>[2x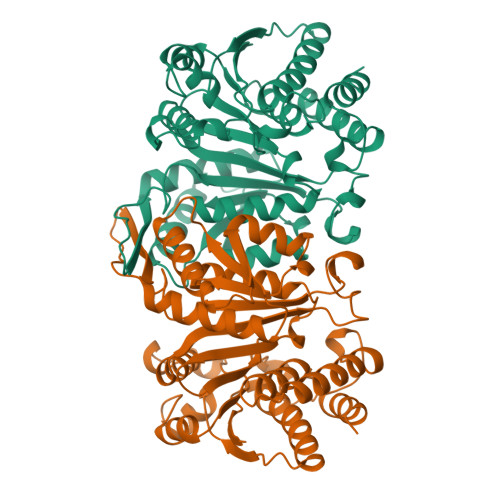]MKVAVLPGDGIGPEVTEAALKVLRALDEAEGLGLAYEVFPFGGAAIDAFGEPFPEPTRKGVEEAEAVLLGSVGGPKWDGLPRKIRPETGLLSLRKSQDLFANLRPAKVFPGLERLSPLKEEIARGVDVLIVRELTGGIYFGEPRGMSEAEAWNTERYSKPEVERVARVAFELARKRRKHVVSVDKANVLEVGEFWRKTVEEVGRGYPDVALEHQYVDAMAMHLVRSPARFDVVVTGNIFGDILSDLASVLPGSLGLLPSASLGRGTPVFEPVHGSAPDIAGKGIANPTAAILSAAMMLEHAFGLVELARKVEDAVAKALLETPPPDLGGSAGTEAFTATVLRHLA> DDLYEEVL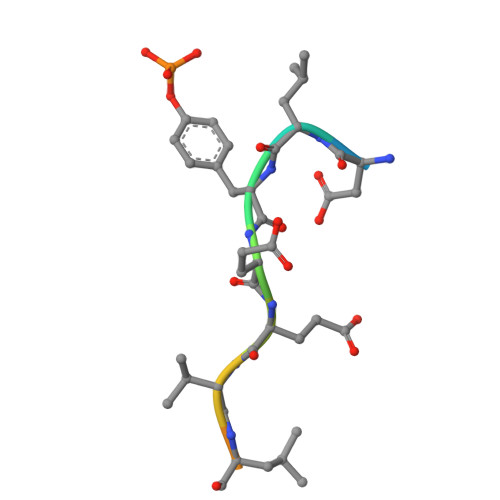FPRN>[2x]MQIGFNFTLTGTLDMVQQMIKERKIDYVEMLIDNFVHLPPEQIADSFDCPVAFHIM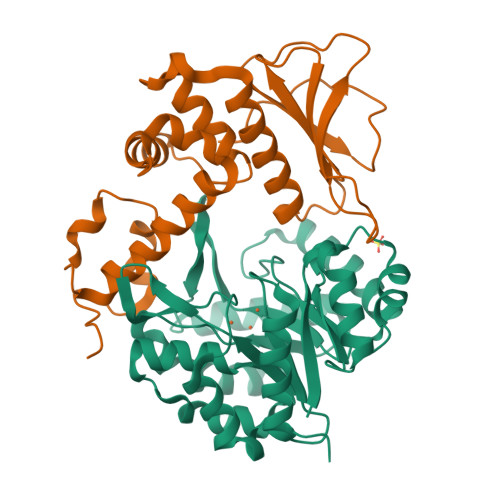LSKYLERDREALAALGKRLRRFIDVMRPVYVSDHILYFTHNGRSLFHLGEIDYGEYDHVRSKVEQWQDMLGTRLYLENYPSIMDGAWDAPSFYERLSRETGVGVLFDASNAICAQNNTGAPVELWKKIIETTRHFHVAGYGTAFIEPRVKADTHDREMAEDTLDFLSRMRTSFDKPGATITYERDFDIDYESISVDLKRLRDIFPCVEEERH;>[2x]MSLLPTAPVRIDADLYDDLANPARQSLYPRDSRGFIRIDISLRAYWHTLFDTCPRLLELSGPSGGAIFLPFMAWARENNLAFDWSFFLWVYVWLQQSEFRERLDEDQLLPVMTASATRWLMIDRDIDACQIVLGSRSLAGAAVVGAKIDSIHCRLEQVQQVAFAAPLPLPDGEFGYFLTPGFEIDHFPGWRPLPR> GGGRGRLILEHTLQGHKGRIWGVAWHPKGNVFASCGEDKAIRIWSLTGNTWSTKTILSDGHKRTIREIRWSPCGQYLASASFDATTAIWSKSSGEFECNATLEGHENEVKSVSWSRSGGLLATCSRDKSVWIWEVAGDDEFECAAVLNPHTQDVKRVVWHPTKDILASASYDNTIKMFAEEPIDNDWDCTATLTSHTSTVWGIDFDADGERLVSCSDDTTIKIWRAYHPGNTAGVATPDQQTVWKCVCTVSGQHSRAIYDVSWCKLTGLIATACGDDGIRIFKESSDSKPDEPTFEQITAEEGAHDQ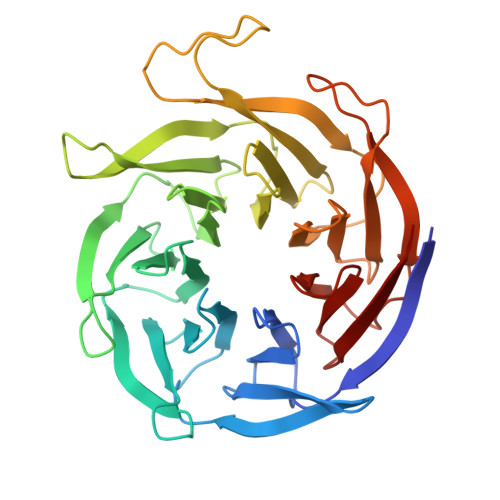DVNSVQWNPVVAGQLISCSDDGTIKIWKVTE>[4x]SNAMSAVMTPAGFTDYKVADITLAAWGRRELIIAESEMPALMGLRRKYAGQQPLKGAKILGCIHMTIQTGVLIETLVALGAEVRWSSCNIFSTQDQAAAAIAAAGIPVFAWKGETEEEYEWCIEQTILKDGQPWDANMVLDDGGDLTEILHKKYPQMLERIHGITEETTTGVHRLLDMLKNGTLKVPA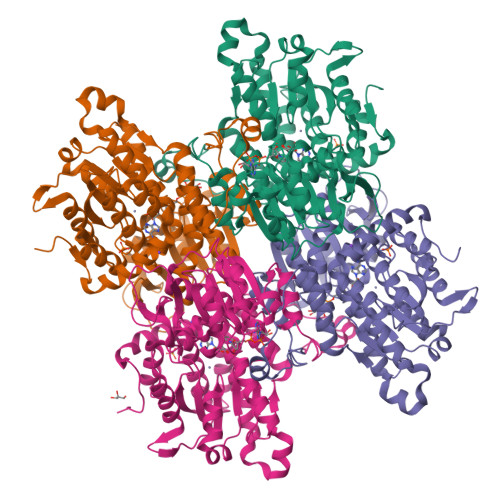INVNDSVTKSKNDNKYGCRHSLNDAIKRGTDHLLSGKQALVIGYGDVGKGSSQSLRQEGMIVKVAEVDPICAMQACMDGFEVVSPYKNGINDGTEASIDAALLGKIDLIVTTTGNVNVCDANMLKALKKRAVVCNIGHFDNEIDTAFMRKNWAWEEVKPQVHKIHRTGKDGFDAHNDDYLILLAEGRLVNLGNATGHPSRIMDGSFANQVLAQIHLFEQKYADLPAAEKAKRLSVEVLPKKLDEEVALEMVKGFGGVVTQLTPKQAEYIGVSVEGPFKPDTYRY> METKTLIVNGMARRLLVSPNDLLVDVLRSQLQLTSVKVGCGKGQCGACTVILDGKVVRACIIKMSRVAENASVTTLEGIGAPDCLHPLQHAWIQHGAAQCGFCTPGFIVSAKALLDENVAPSREDVRDWFQKHHNICRCTGYKPLVDAVMDAAAILRGEKTVEEISFKMPADGRIWGSSIPRPSAVAKVTGLAEFGADAALRMPENTLHLALAQAKVSHALIKGIDTSEAEKMPGVYKVLTHKDVKGKNRITGLITFPTNKGDGWERPILNDSKIFQYGDALAIVCADSEANARAAAEKVKFDLELLPEYMSAPEAMAPDAIEIHPGTPNVYYDQLEEKGEDTVPFFNDPANVVAEGSYYTQRQPHLPIEPDVGYGYINEQGQVVIHSKSVAIHLHALMIAPGLGLEFPKDLVLVQNTTGGTFGYKFSPTMEALVGVAVMATGRPCHLRYNYEQQQNYTGKRSPFWTTMRYAADRQGKILAMETDWSVDHGPYSEFGDLLTLRGAQYIGAGYGIANIRGTGRTVATNHCWGAAFRGYGAPESEFPSEVLMDELAEKLGMDPFELRALNCYREGDTTSSGQIPEVMSLPEMFDKMRPYYEESKKRVKERSTAEIKRGVGVALGVYGAGLDGPDTSEAWVELNDDGSVTLGNSWEDHGQGADAGSLGTAHEALRPLGITPENIHLVMNDTSKTPNSGPAGGSRSQVVTG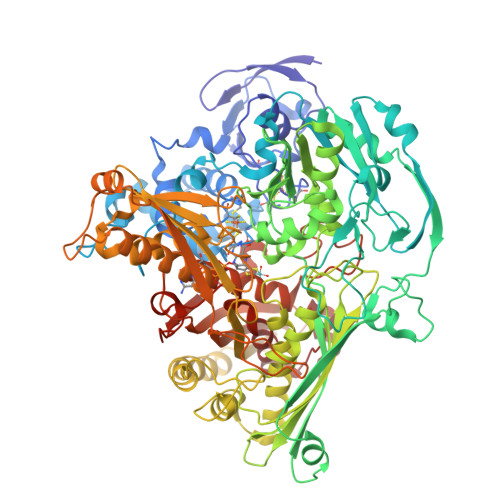NAIRVACEMLIEGMRKPGGGFFTPAEMKAEGRPMRYDGKWTAPAKDCDAKGQGSPFACYMYGLFLTEVAVEVATGKATVEKMVCVADIGKICNKLVVDGQIYGGLAQGVGLALSEDYEDLKKHSTMGGAGIPSIKMIPDDIEIVYVETPRKDGPFGASGVGEMPLTAPHAAIINGIYNACGARVRHLPARPEKVLEAMPR> SEDDGSASPESQEMSYTELPCPSICPLIYAPVCVEDSNQDFYLFVNECEVRKCGCEAGFV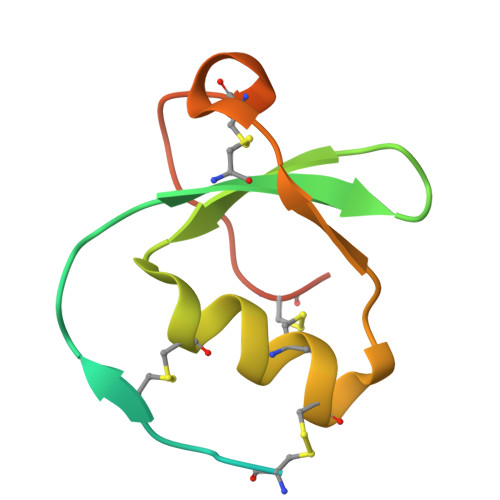YTFVPREMCKATTSLCPMQTKSS> NPVERYVDEVLNEVLVVPNINQSHPTTSNAAPVLDAAETGHTNKIQPEDTIETRYVQSSQTLDEMSVESFLGRSGCIHESVLDIVDNYNDQSFTKWNINLQEMAQIRRKFEMFTYARFDSEITMVPSVAAKDGHIGHIVMQYMYVPPGAPIPTTRDDYAWQSGTNASVFWQHGQPFP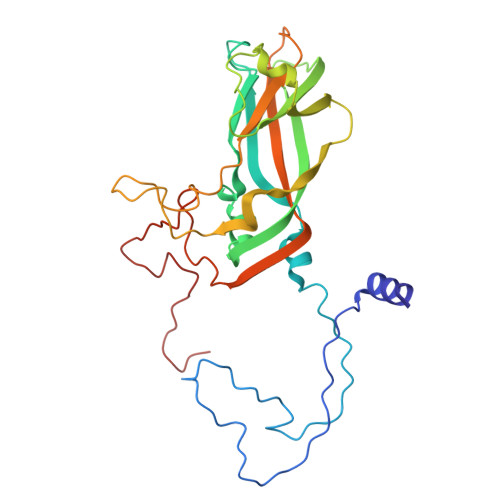RFSLPFLSIASAYYMFYDGYDGDTYKSRYGTVVTNDMGTLCSRIVTSEQLHKVKVVTRIYHKAKHTKAWCPRPPRAVQYSHTHTTNYKLSSEVHNDVAIRPRTNLTTV> SKAKDLASLPEIKSQGYHILFGELRDGEYTEGKILVGYNDRSEVDKIVKAVNGKVVLELPQIKVVSIKLNGMTVKQAYDKIKALALKGIRYVEPSYKRELIKPTVVKPNPDMYKIRKPGLNSTARDYGEELSNELWGLEAIGVTQQLWEEASGTNIIVAVVDTGVDGTHPDLEGQVIAGYRPAFDEELPAGTDSSYGGSAGTHVAGTIAAKKDGKGIVGVAPGAKIMPIVIFDDPALVGGNGYVGDDYVAAGIIWATDHGAKVMNHSWGGWGYSYTMKEAFDYAMEHGVVMVVSAGNNTSDSHHQYPAGYPGVIQVAALDYYGGTFRVAGFSSRSDGVSV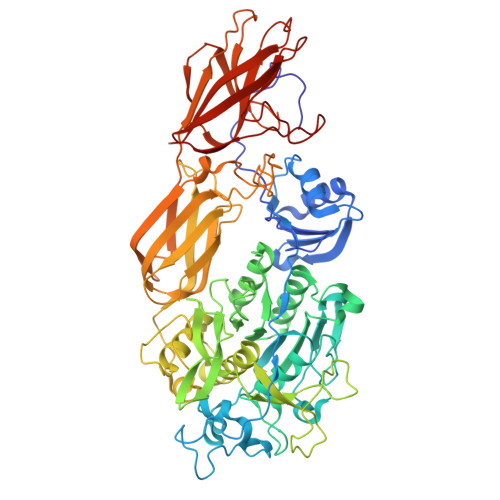GAPGVTILSTVPGEDSIGYEGHNENVPATNGGTYDYYQGTSMAAPHVTGVVAVLLQKFPNAKPWQIRKLLENTAFDFNGNGWDHDTGYGLVKLDAALQGPLPTQGGVEEFQVVVTDAKGNFGVPTVFVSMMRDNGSCYYAKTGPDGIARFPHIDSGTYDIFVGGPDHWDRALAPYDGESIPGGYAIALRMAEERQASFVGFGVSPDATQLNVNFNSTLQVKFSTNLSTLKDPQFVVVDPLLRGVYGRVAYARNQTYDLSLLSGQISFGIQTLLPAATDITIQGTVTLNGEDIPVYGVLKAGTTWTIIDDFGGLNLGTDSQPIYVWWTIFGQ> MINGVYYNEISRDLDISSSTQCLRFLKETVIPSLANNGNNSTSIQYHGISKNDNIKKSVNKLDKQINMADRSLGLQQVV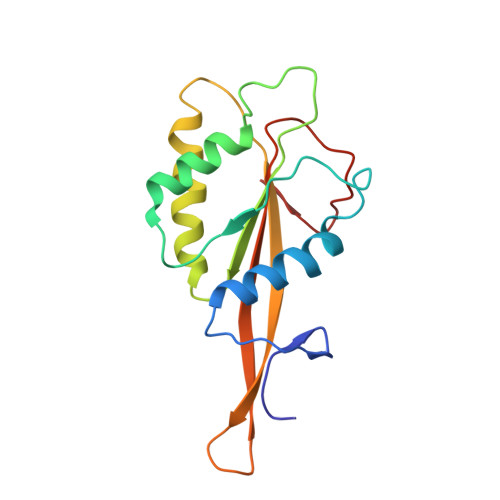CIFSYGPHIQKMLSILEIFKKGYIKNNKKIYQWNKLTSFDIKREGRNELQEERLKVPILVTLVSDSEIIDLNLHSFTKQ> MHHHHHHENLYFQSMPVEEPLATLSSIPDSSADQAPPLIADEFTLDLPRIPSLELPLNVSTKHSSIQKAIKMCGGIEKVKEAFKEHGPIESQHGLQLYLNDDTDSDGSKSYFNEHPVIGKRVPFRDESVILKVTMPKGTLSKNNNSVKDSIKSLKDSNKLRVTPVSIVDNTIKFREMSDFQIKLDNVPSAREFKSSFGSLEWNNFKSFVN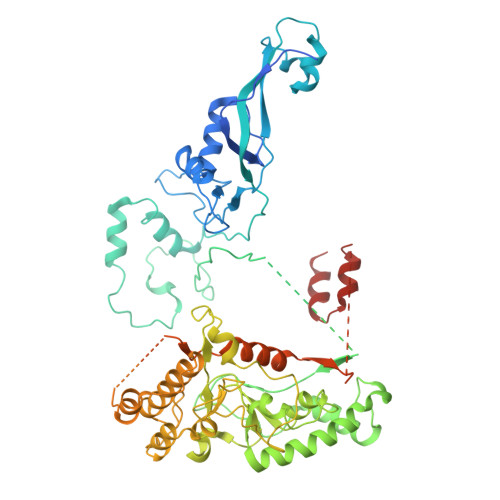SVPDNDSQPQENIGNLILDRSVKIPSTDFQLPPPPKLSMVGFPLLYKYKANPFAKKKKNGVTEVKGTYIKNYQLFVHDLSDKTVIPSQAHEQVLYDFEVAKKTKVYPGTKSDSKFYESLEECLKILRELFARRPIWVKRHLDGIVPKKIHHTMKIALALISYRFTMGPWRNTYIKFGIDPRSSVEYAQYQTEYFKIERKLLSSPIVKKNVPKPPPLVFESDTPGGIDSRFKFDGKRIPWYLMLQIDLLIGEPNIAEVFHNVEYLDKANELTGWFKELDLVKIRRIVKYELGCMVQGNYEYNKYKLKYFKTMLFVKESMVPENKNSEEGMGVNTNKDADGDINMDAGSQMSSNAIEEDKGIAAGDDFDDNGAITEEPDDAALENEEMDTDQNLKVPASIDDDVDDVDADEEEQESFDVKTASFQDIINKIAKLDPKTAETMKSELKGFVDEVDLXXXXXXXXXXXXXXXXXXXXXX> SQLPPGKPEIFKCRSPNKETFTCWWRPGTDGGLPTNYSLTYHREGETLMHECPDYITGGPNSCHFGKQYTSMWRTYIMMVNATNQMGSSFSDELYVDVTYIVQPDPPLELAVEVKQPEDRKPYLWIKWSPPTLIDLKTGWFTLLYEIRLKPEKAAEWEIHFAGQQTEFKILSLHPGQKYLVQVRCKPDHGYWSAWSPATFIQIPSDF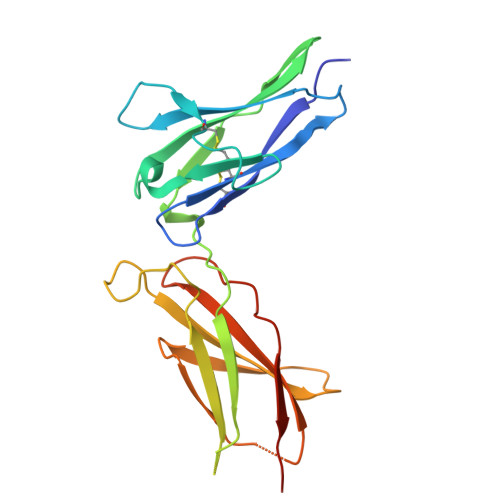TMND>MSRAAQLLPGTWQVTMTNEDGQTSQGQMHFQPRSPYTLDIVAQGTISDGRP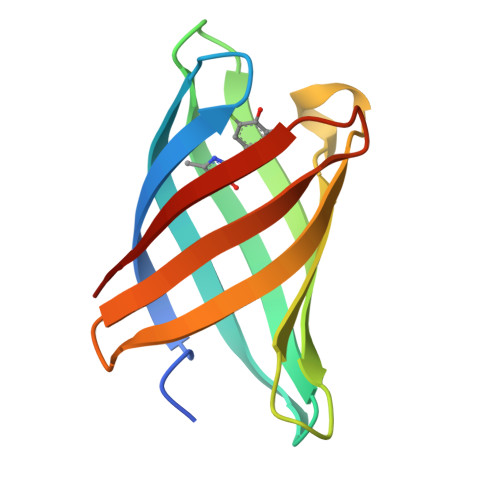ITGYGKVTVKTDDTLHVNITYPSLGNIKVQGQITMDSPTQATWNSTTSDGKKLTGTLQRQE[2x]>[2x]MKKIYKQISGALLMLTLILNITACSPESFTSPNEAGIPVVSDYEDCIRIDVNQETNYVTFSFQGQKGVMPIWIIDGKNYSSSFNMTKYYRKAGDYSVEVKIANSNGVSDRAITRNFHIDKTIMTGFGGFDPESNFNIWRTATISEPTFWYAPGWSQIADPAYSLVNGTYTVTLPEATSETWQAQMPIKTNIATDAGKNYDFSVILTSTIDHPNVTVKLVDATE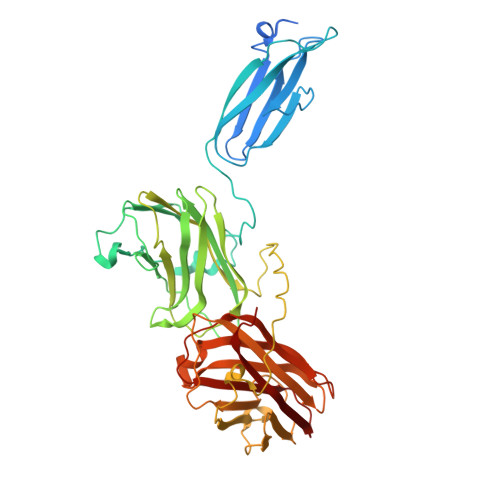DKIYYFEGKTPLVANEPVCFWKSNMPGLDIANLNLVFDFGGNAAGTVMTIESIVLKDHANDDGTIVPEQEETPEPTWSAVDSEDNLWHSVTFTNEFYYAPGWNPIANPALNIDGATYTLNFPTATNEKWQNQVTFISDALTASAEENYDFRVILNASNDISSATIKLVQVGGGDNDNIFVFLLEDVKLTAGEDVTAKVINAKGVDITQAKLVFDFGGNPANTEVIIKDIILQKHKD> MGGEALTLPKDLLDFSGYGPKELQALLDLAEQLKR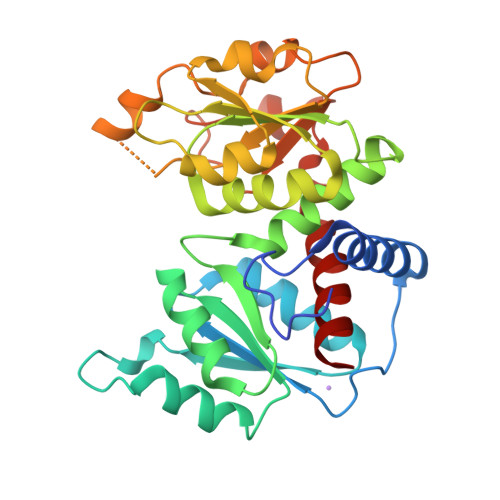ERYRGEDLKGKVLALLFEKPSLRTRTTLEVAMVHLGGHAVYLDQKQVGIGEREPVRDVAKNLERFVEGIAARVFRHETVEALARHAKVPVVNALSDRAHPLQALADLLTLKEVFGGLAGLEVAWVGDGNNVLNSLLEVAPLAGLKVRVATPKGYEPDPGLLKRANAFFTHDPKEAALGAHALYTDVWTSMGQEAEREKRLRDFQGFQVNGELLKLLRPEGVFLHCLPAHYGEETTEEAVHGPRSRVFDQAENRLHTAKAVLLTLLK> GGLEKDFLP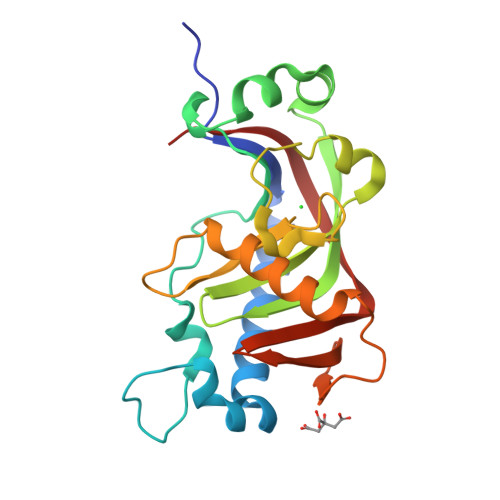LYFGWFLTKKSSETLRKAGQVFLEELGNHKAFKKELRHFISGDEPKEKLELVSYFGKRPPGVLHCTTKFCDYGKAAGAEEYAQQEVVKRSYGKAFKLSISALFVTPKTAGAQVVLTDQELQLWPSDLDKPSASEGLPPGSRAHVTLGCAADVQPVQTGLDLLDILQQVKGGSQGEAVGELPRGKLYSLGKGRWMLSLTKKMEVKAIFTGYYG>PLGSVSEACPVCEKTVQNPCVLETGYVACYPCAISYLVNNEGHCPVTNKKLLGCTYNKHTNKWEVVTGIRKLI[2x]

Luminal peroxisomal proteins are imported from the cytosol by mobile receptors, which then recycle back to the cytosol by a poorly understood process. Recycling requires receptor modification by a membrane-embedded ubiquitin ligase complex comprising three RING finger domain-containing proteins (Pex2, Pex10 and Pex12). Here we report a cryo-electron microscopy structure of the ligase complex, which together with biochemical and in vivo experiments reveals its function as a retrotranslocation channel for peroxisomal import receptors. We propose that the N terminus of a recycling receptor is inserted from the peroxisomal lumen into the pore and monoubiquitylated by RF2 to enable extraction into the cytosol.

By contrast, neither RF2 nor RF12 is a canonical ring finger. RF12 deviates even more from canonical ring fingers. It contains only five, instead of seven, conserved Cys residues, and lacks the second Zn2+ atom, as seen in both the cryo-EM structure and a crystal structure of the S. cerevisiae homologue that we determined at 1.5 Å resolution. RF12 is therefore not predicted to interact with an E2 enzyme. The structural features of the ring finger domains are consistent with results of an in vitro polyubiquitylation assay that uses isolated ring fingers and the E2 enzyme Ubc4. RF10 has some low activity, whereas both RF2 and RF12 are inactive (lane 4 and Extended Data Fig. 8a). RF12 is an activator of RF10, as it greatly stimulated the polyubiquitylation by RF10 (lane 5), in agreement with previous results. Mutation of L398 considerably reduced the stimulatory effect of RF12 in the in vitro assay. Thus, RF10 and RF12 probably function as a unit in polyubiquitylation.>GMPLTGEYEPSPSDWARKQVETYENSGGTEGTTLQGK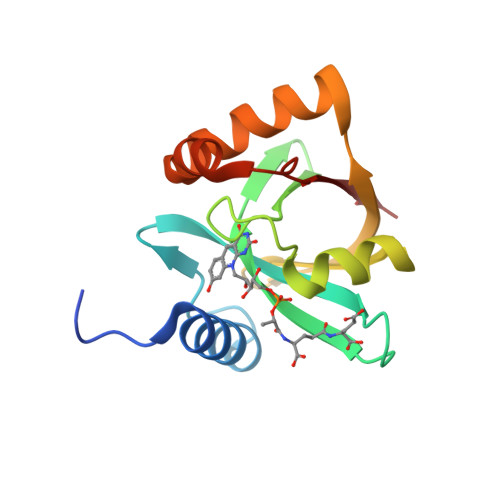PVVVLTTKGAKTGKLRKTPLMRVEHNGEYAVVASLGGAPKHPVWYHNIKAEPHVELRDGTEVGDYTAREVTGEEKRVWWERAVEVWPDYAEYQTKTTREIPVFVLTPR[2x]> MGGKGLNNCVFSYLPSYGDDEVSVYHPICEAALNQALVNTGLDSTYEVVHHELVGSIEADFVIKNKQTKKYLLIVEVKRTKSQVSSTRYRLQAQSYVREANIKVEQHYYCLTNLEIIDFFKHDPNKPVVSQQIIEPSPIVVGNFSDTVSEFYNRLVEAFQNIIDISVNDAGTYKSSTANLVDILENRKDNSTSWHQALVVAGYEYIRGVLRGQNVEVPTRDAIYFKSRPGRLLEEGRKIDFNVLFSEPEPNTNDNDIWNVNLLSSLND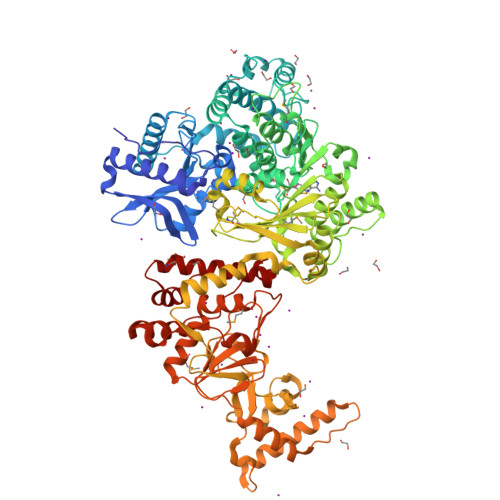LGRRILTGDELAELIHDIATRGRGHEGVVPTDIELGKVLSIISQHILGRPLTEDEVISDPAAGSGNLLATVSAGFNNVMPRQIWANDIETLFLELLSIRLGLLFPQLVSSNNAPTITGEDVCSLNPEDFANVSVVVMNPPYVSGVTDPAIKRKFAHKIIQLTGNRPQTLFGQIGVEALFLELVTELVQDGTVISAIMPKQYLTAQGNESKAFREFLVGNFGLEHIFLYPREGLFEEVIKDTVVFVGRKGSSVEEIEVLDSFTPLEQVDLHNLKRALSNSSNEQIIQPMGMELRKEKREELENRVTVGWRHITSNGRVAEEWITNNLESHCIRLVASDYDLRRGRVGNKGASDLLFINSKKKLWDLLDESVPRDWLYPALRKVNEINTPIFNEDATPVRFLCPPNSAYQDGTGESIILDKILDVYVDFQVYKSKQKKFEKSKEELKEILYKESDFYSSEHTVFIPRALRRSARAFINEQKVFCSTNALEVFGGNSEEMWLLLSWLSSVFAQLQFEAMAKDQEGERKLEKKSIQNLYIPNLGDIDDVLKQDLIEEVREIHFFDLCRPRVRKLDLLWAKVFWSGNEMSKTKEAAELLEDLVFERYPEGSQIGE> MAFCIAVIGKDNAPLYLTTSDMEQELELQYHVNAALDVVEEKCLIGKG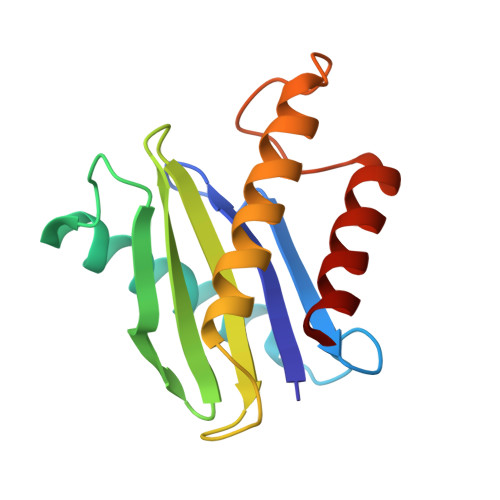APESKELYLGLLYSTENHKIYGFVTNTRVKFIVVIDSSNVALRENEVRAIFRNLHLLYTDAICNPFYIPGESLTSKKFDRAVQKLMSGTA>[4x]MKNYQKMSVAQDARVELHDSLALTGAEVSINHLPAGAGVPFVHSHKQNEEIYGILSGKGFITIDGEKIELQAGDWLRIAPDG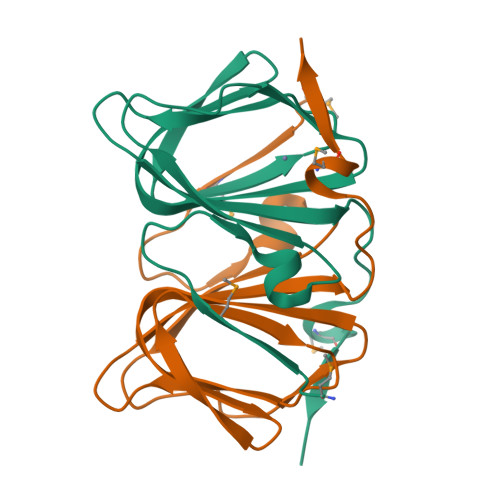KRQISAASDSPIGFLCIQVKAGSLEGYTMTDGVVQLEHHHHHH2-{(R)-(3-{[(2E)-4-(dimethylamino)but-2-enoyl]amino}phenyl)[2-(piperidin-1-yl)ethoxy]methyl}thieno[3,2-b]pyridine-7-carboxylic 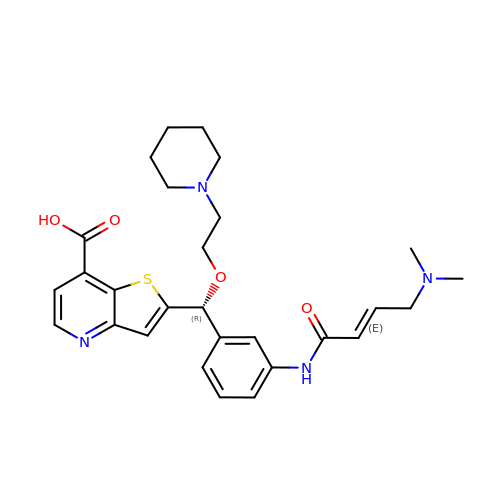acid | C28 H34 N4 O4 S | KIIDGZQVWULCMZ-GYAHLDOBSA-N cis-4-{[2-({4-[(1E)-3-morpholin-4-yl-3-oxoprop-1-en-1-yl]-2,3-bis(trifluoromethyl)phenyl}sulfanyl)phenoxy]methyl}cyclohexanecarboxylic 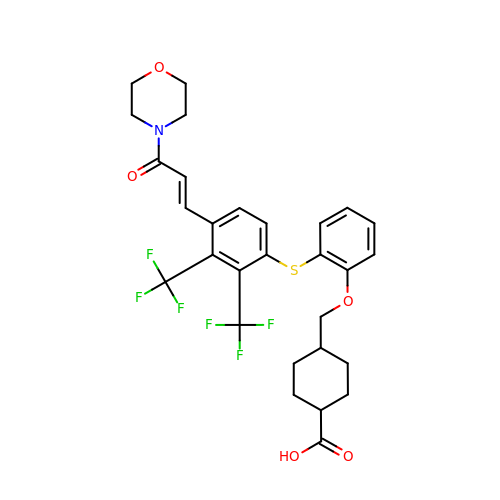acid | C29 H29 F6 N O5 S | AXSOGTWJBSDWJQ-WZEPYWGYSA-N> GSGPIQLWQFLLELLTDKSCQSFISWTGDGWEFKLSDPDEVARRWGKRKNKPKMNYEKLSRGLRYYYDKNIIHKTAGKRYVYRFVCDL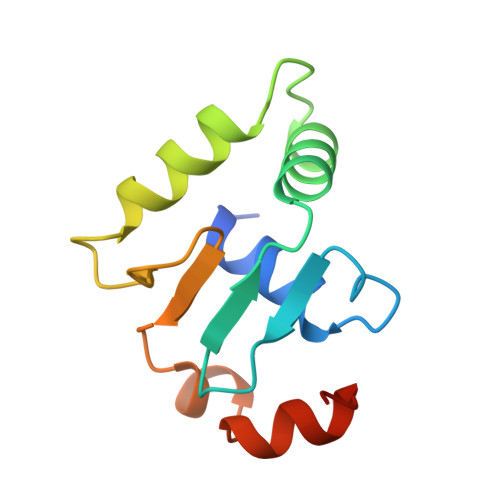QSLLGYTPEELHAMLDVKPDAD> MANGNEGLSTTTKYIFVPIATIGCGKTTVFNTLNNLFPQWTHIQNDNISKKAKLKICDLTLLALEDDD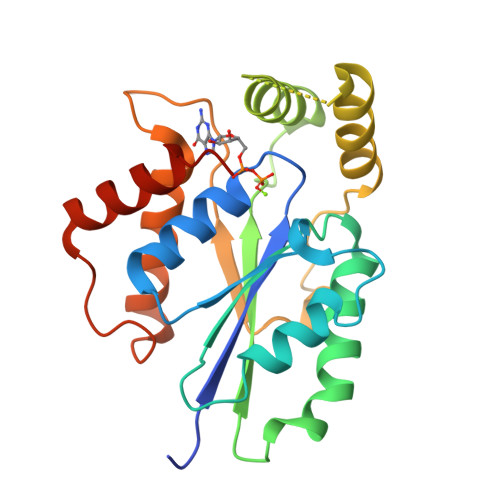QSVVLFDRNNSASRERRQIFTTIDQKRDEHLDDTVDLKYIAINFIPEDLSEEELWDITYNRVIQRGDNHQSIKSQLDENLVESVMKGFIQRYQPINTSRSPDDQFDHVIHLKLSKDENSSKSSLENVRIIIDDLVQNFPDLIKEKPADELINECFQKALDYKPTFVKN6-CHLORO-2-(1-FURO[2,3-C]PYRIDIN-5-YL-ETHYLSULFANYL)-PYRIMIDIN-4-YLAMINE 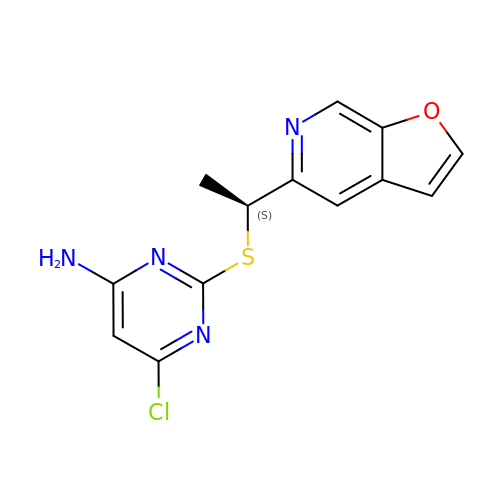| C13 H11 Cl N4 O S | ATCRIOJPQXDFNY-ZETCQYMHSA-N>[2x]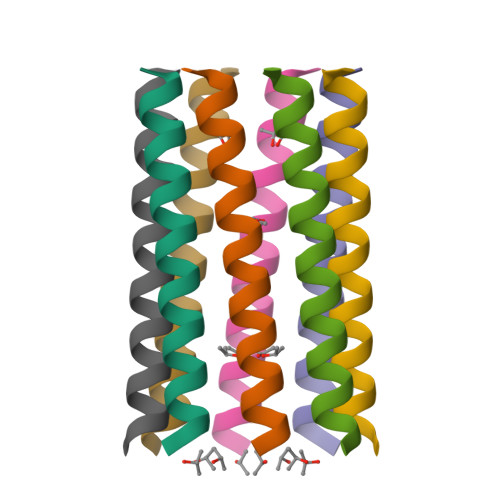XGEIAQALKEIAKALKEIAWALKESAQALKGX>HHHHHHGGAMNIQALLSEKVRQAMIAAGAPADCEPQVRQSAKVQFGDYQANGMMAVAKKLGMAPRQLAEQVLTHLDLNGIASKVEIAGPGFINIFLDPAFLAEHVQQALASDRLGVATPEKQTIVVDYSAPNVAKEMHVGHLRSTIIGDAAVRTLEFLGHKVIRANHVGDWGTQFGMLIAWLEKQQQENAGEMELADLEGFYRDAKKHYDEDEEFAERARNYVVKLQSGDEYFREMWRKLVDITMTQNQITYDRLNVTLTRDDVMGESLYNPMLPGIVADLKAKGLAVESEGATVVFLDEFKNKEGEPMGVIIQKKDGGYLYTTTDIACAKYRYETLHADRVLYYIDSRQHQHLMQAWAIVRKAGYVPESVPLEHHMFGMMLGKDGKPFKTRAGGTVKLADLLDEALERARRLVAEKNPDMPADELEKLANAVGIGAVKYADLSKNRTTDYIFDWDNMLAFEGNTAPYMQYAYTRVLSVFRKAEIDEEQLAAAPVIIREDREAQLAARLLQFEETLTVV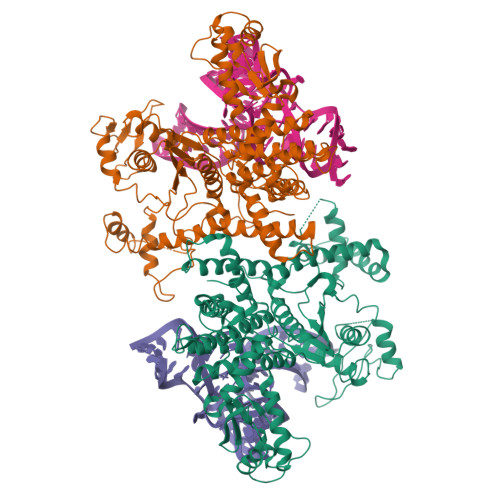AREGTPHVMCAYLYDLAGLFSGFYEHCPILSAENEEVRNSRLKLAQLTAKTLKLGLDTLGIETVERMR[2x]>MMSEIIAVANQKGGVGKTTTAVNLAASLAVHEKKILLIDFAPQANATSSLGFRRDKIDYDIYHVLIGRKQISQVILKTQMPFLDLVPSNLGLAGFEKTFYDSQDENKRGELMLKNALESVVGLYDYIIIDSPPALGPLTINSLSAAHSVIIPIQCEFFALEGTKLLLNTIRMLQKSTNPKLKIRGFLPTMHVPQLNLTKGVLAELFKYFDSEFFRDSATGEYIMIPKSVKLAESPSFGKPILLYDIKSNGSIAYQKLAQSILQG[4x];>MAKNKVLGRG[4x]

The ParABS system, composed of ParA (an ATPase), ParB (a DNA binding protein), and parS (a centromere-like DNA), regulates bacterial chromosome partition. In Helicobacter pylori, ParA and ParB homologs are encoded as HpSoj and HpSpo0J (HpParA and HpParB), respectively. ParA forms as a dimer in the ATP-bound state that can bind to nsDNA through a continuous basic binding patch formed by arginine/lysine residues. The partition complex interacts with the nucleoid-bound ParA forming the nucleoprotein ParA–ParB–DNA complex, known as the nucleoid–adaptor complex (NAC).

To investigate the molecular mechanism of NAC formation, we determined the crystal structure of the HpParAD41A–DNA in complex with residues 1–10 (1MAKNKVLGRG10) of the HpParB N-terminus (HpParBN10), referred to as the HpParAD41A–DNA–HpParBN10 complex. The overall structure revealed that one HpParAD41A dimers binds to one 24-bps DNA, exhibiting the same architecture as the HpParAD41A–DNA complex. Additionally, each HpParAD41A binds to one HpParBN10 peptide, as confirmed by the electron density map. The HpParBN10 is located near the dimer interface but is inclined towards two loops, loop α2α3 (L23) and β3β4 (L34). The HpParBN10 is clamped by the two flexible loops, L23 and L34, of HpParAD41A. Moreover, Arg9 is oriented towards the phenyl group of HpParAD41A Phe52, forming a specific cation-π interaction between the amino group and the phenyl group. Furthermore, the main chain of HpParBN10 Arg9 interacts with HpParAD41A Gln79 at L34, providing an additional interaction that stabilizes the HpParBN10. When superimposing the four protomers of the asymmetry unit in the HpParAD41A-DNA-HpParBN10 complex, only HpParBN10 Arg9 is located precisely in the same position, while the remaining part of HpParBN10 exhibits different conformations due to the peptide's flexibility. The binding of HpParBN10 may not affect the formation of the ATP-sandwich dimer or the HpParA-DNA complex. The HpParAD41A-DNA-HpParBN10 complex represents the first ParA, ParB and DNA ternary complex (NAC) within the ParABS superfamily.> ASTLKSGSKEVENLKKPFMPPREVHVQVTHSMPPQKIEIFKSLDNWAEENILVHLKPVEKCWQPQDFLPDPASDGFDEQVRELRERAKEIPDDYFVVLVGDMITEEALPTYQTMLNTLDGVRDETGASPTSWAIWTRAWTAEENRHGDLLNKYLYLSGRVDMRQIEKTIQYLIGSGMDPRTENSPYLGFIYTSFQERATFISHGNTARQAKEHGDIKLAQICGTIAADEKRHETAYTKIVEKLFEIDPDGTVLAFADMMRKKISMPAHLMYDGRDDNLFDHFS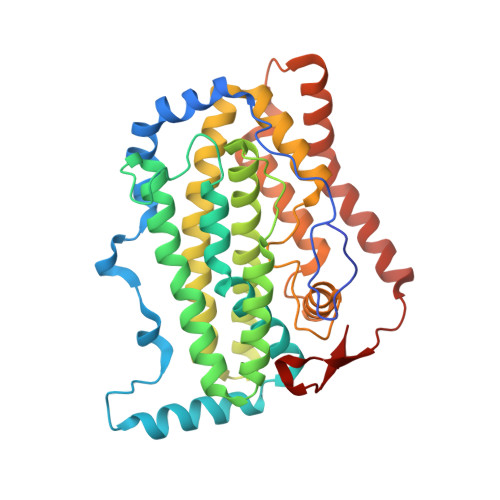AVAQRLGVYTAKDYADILEFLVGRWKVDKLTGLSAEGQKAQDYVCRLPPRIRRLEERAQGRAKEAPTMPFSWIFDRQVKL>TPQNITDLCAEYHNTQIYTLNDKIFSYTESLAGKREMAIITFKN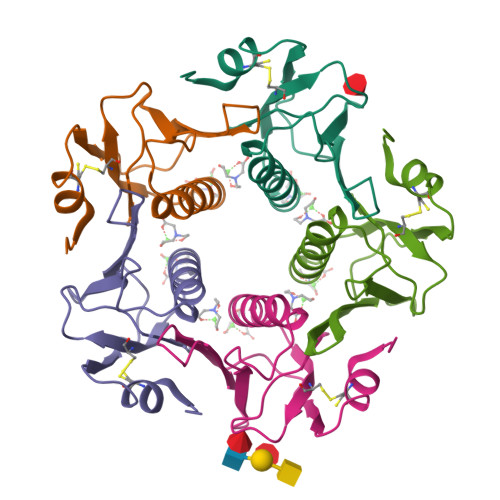GAIFQVEVPGSQHIDSQKKAIERMKDTLRIAYLTEAKVEKLCVWNNKTPHAIAAISMAN[10x]>MSSTFEPATDSPLPVPGVQYFLQHVQSGKYVHPHGGSDM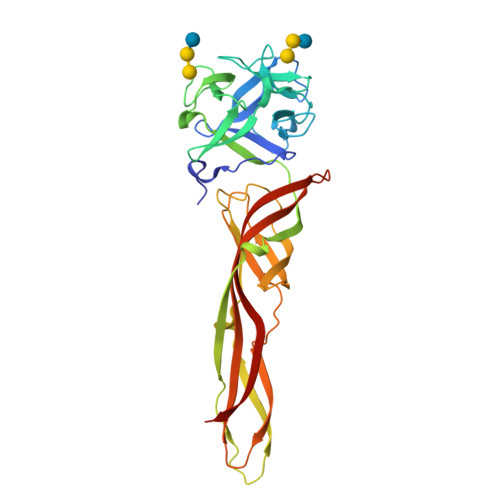PGNDTALVLHHGFDEKRDALRWVFVNDAENKHQLKHYSSGKFVHPKGGKVGKEATLVVHSSPGRPETMIEMVQEDGRTYLRHTDSDYYVHPHGGSPNPGDNTRLVYYSGYRPSLAFLAIPAETLFVDRIEIHQAQALESINTITSLSDEHRNDTDQPVQTSISVALEESLQDSAQLSFERCFGLKVGSEFEVGLPLVGKTKVSVQFSGSWKSSTIKGEVRTSAVKVQINEHVTIPPGKCVQIRIDTRRCTKTAPATMYLRTASGIEVQRETTVTSTYHYDQEVHVVPVTN[2x]>[2x]MTERIRNVALRSKVCPAETASELIKHGDVVGTSGFTGAGYPKEVPKALAQRMEAAHDRGEKYQISLITGASTGPQLDGELAKANGVYFRSPFNTDATMRNRINAGETEYFDNHLGQVAGRAVQGNYGKFNIALVEATAITEDGGIV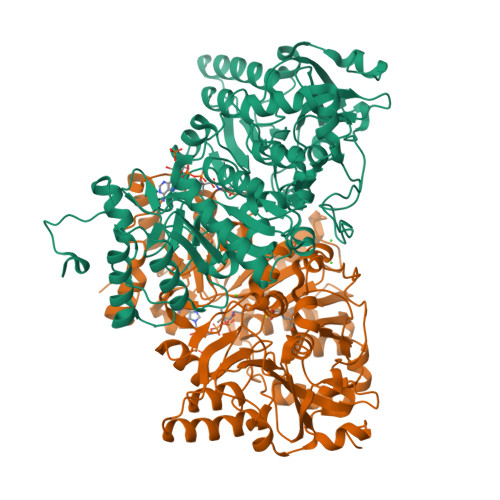PTSSVGNSQTFLNLAEKVIIEVNEWQNPMLEGIHDIWDGNVSGVPTRDIVPIVRADQRVGGPVLRVNPDKIAAIVRTNDRDENAPFAAPDETAKAIAGYLLDFFGHEVKQNRLPPSLLPLQSGVGNVANAVLEGLKEGPFENLVGYSEVIQDGMLAMLDSGRMRIASASSFSLSPEAAEEINNRMDFFRSKIILRQQDVSNSPGIIRRLGCIAMNGMIEADIYGNVNSTRVMGSKMMNGIGGSGDFARSSYLSIFLSPSTAKGGKISAIVPMAAHVDHIMQDAQIFVTEQGLADLRGLSPVQRAREIISKCAHPDYRPMLQDYFDRALKNSFGKHTPHLLTEALSWHQRFIDTGTMLPSSLEHHHHHH> MWELRSASFWRAICAEFFASLFYVFFGLGASLRWAPGPLHVLQVALAFGLALATL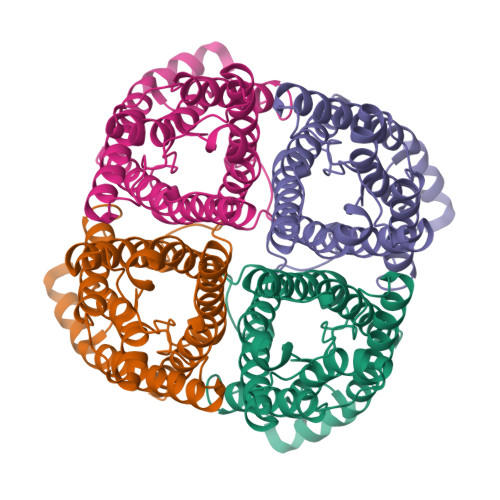VQAVGHISGAHVNPAVTFAFLVGSQMSLLRAICYMVAQLLGAVAGAAVLYSVTPPAVRGNLALNTLHPGVSVGQATIVEIFLTLQFVLCIFATYDERRNGRLGSVALAVGFSLTLGHLFGMYYTGAGMNPARSFAPAILTRNFTNHWVYWVGPVIGAGLGSLLYDFLLFPRLKSVSERLSILKGSRPSESNGQPEVTGEPVELKTQAL> MPLARIPRARRAVATLVGLAATVLLTAAAVPSADAGRPAYRDPRLPVPDRVDDLMARMSLDDKLGQMVQVERKAAGPQAVADHRIGSVLSGGGSAPEPNTPQAWADMYDSYQRAALSTPLGIPLIYGVDAVHGHNNVHGATIYPHNIGLGATGNPDLVQRIGAATAE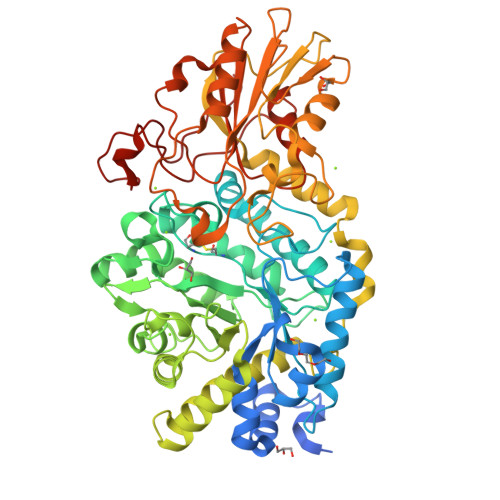EVAATGIDWSFAPCVCVARDDRWGRTYESFGEKSENASAMTSAVTGLQGEALGATPSSVMATAKHYVGDGGTTGGDDQGNTEISEQELREIHLPPFREAIARGVGSVMVSYSSWNGEKLHASTYLVNDVLKGELGFTGLVVSDYDAIDKLDGQEDFTPDEVRASVNAGIDMFMMSSRHEKFIDYLRAEVEAGRVPAERIDDANRRILTKKFELGLFERPFAQRDLLPTVGSAEHRELARQAVRESQVLLRNDGVLPLAKDGGKLFVAGKNADDIGNQSGGWTISWQGSSGDITEGTTILEGIRAAASGSEVTYDRHGNGVDGSYRAAIAVVGETPYAEFEGDRPGGLGLDEEDRATIAKLRASGVPVVVVTVSGRPLDIAGEVDGWNALLASWLPGSEGQGVADVLFGDHNPTGKLPMTWMRSFDQLPINDGDGQDPLFPHGFGLSYG> GPGSEFRQDKMREEGLQLVSMIREGEAAGACPEEIFSALQYSGTEVPLQWLRSELPYVLEMVAELAGQQDPGLGAFSCQEARRAWLDRHGNLDEAVEECVRTRRRKVQELQSLGFGPEEGSLQALFQHGGDVSRALTELQR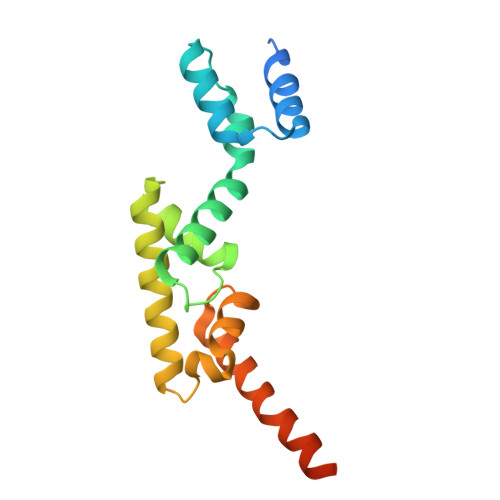QRLEPFRQRLWDSGPEPTPSWDGPD The PH domain-containing protein Slm1 from budding yeast Saccharomyces cerevisiae is required for actin cytoskeleton polarization and cell growth. The PH domain-containing protein Slm1 from S. cerevisiae is a component of the target of rapamycin complex 2 (TORC2) signaling pathway. We have previously reported that in vitro, the Slm1-PH domain (Slm1-PH) interacts with liposomes containing PtdIns(4,5)P2 and DHS-1P cooperatively. The core of each monomer consists of seven antiparallel β-strands with a C-terminal amphipathic α-helix connected via a long and flexible loop.

In summary, here we present the first three-dimensional structures of the Slm1-PH bound to Ins(4)P and phosphoserine and show that the Slm1-PH exhibits a non-canonical PtdInsPs-binding mechanism. The phosphoserine contacts the β1-β2 region and the β5-β6 loop through the same key residues as Ins(4)P. Specifically, the hydroxyl group of Tyr485 hydrogen bonds with the nitrogen atom of phosphoserine (hydrogen bond length  = 2.9 Å) and the NH2 group of Arg478 interacts with the oxygen atom of phosphoserine (hydrogen bond length  = 2.8 Å). In addition, the ε-amino group of Lys542 from the β5-β6 loop and the ε-amino group of Lys562 from the β7-strand also interact with the phosphate group of the phosphoserine molecule (hydrogen bond lengths  = 2.4 Å and 2.7 Å, respectively). In the non-canonical binding site there are four residues that are consistently involved in ligand binding: Arg478, Tyr485, Lys542 and Lys562. The Ins(4)P and phosphoserine molecules superposed well on to the Ins(1,4,5)P3 of the β-spectrin PH complex positioned in the non-canonical binding site. The non-canonical binding site accommodated anions from the crystallization conditions, and also the phosphoserine molecule. In addition, all structures in complex with ligands show regions of additional density between the bottom of the β1-β2 loop and the N-terminus of Slm1-PH. Intriguingly, we could not assign any ligand to these extra densities.

> DHPFTEIKSGFLERRSKFLKSYSKGYYVLTPNFLHEFKTADRKKDLVPVMSLALSECTVTEHSRKNSTSSPNSTGSDAKFVLHAKQNGIIRRGHNWVFKADSYESMMSWFDNLKILTSTS;> DHPFTEIKSGFLERRSKFLKSYSKGYYVLTPNFLHEFKTADRKKDLVPVMSLALSECTVTEHSRKNSTSSPNSTGSDAKFVLHAKQNGIIRRGHNYVFKADSYESMMSWFDNLKILTSTS>MDLADRFAELERRYDARL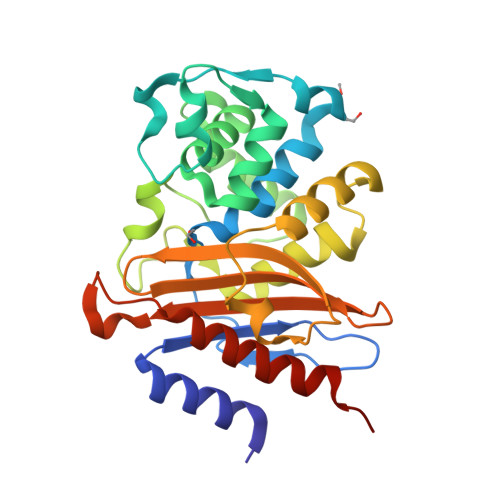GVYVPATGTTAAIEYRADERFAFCCTFKAPLVAAVLHQNPLTHLDKLITYTSDDIRSISPVAQQHVQTGMTIGQLCDAAIRYSDGTAANLLLADLGGPGGGTAAFTGYLRSLGDTVSRLDAEEPELNRDPPGDERDTTTPHAIALVLQQLVLGNALPPDKRALLTDWMARNTTGAKRIRAGFPADWKVIDKTGTGDYGRANDIAVVWSPTGVPYVVAVMSDRAGGGYDAEPREALLAEAATCVAGVLALEHHHHHH[2x]>MKHHHHHHPMAMNLINQKLFDFECDAYHDGEFTRVSTEDILGKWSIFFFYPADF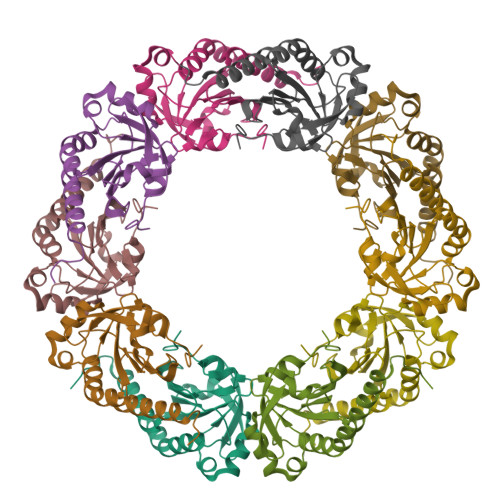SFVCPTELGDMQEHYAHLQELNCEVYSVSEDSHYVHKAWADATETIGKIKYPMLADPNGQLARFFGVLDEASGMAYRASFIVSPEGDIKSYEINDMGIGRNAEELVRKLEASQFVAEHGDKVCPANWQP[5x]>[4x]MRIQVNAKGAARLLSRHLWVFRRDVVSGPETPGLYPVYWGRRFLALALYNPHTDLAVRAYRFAPA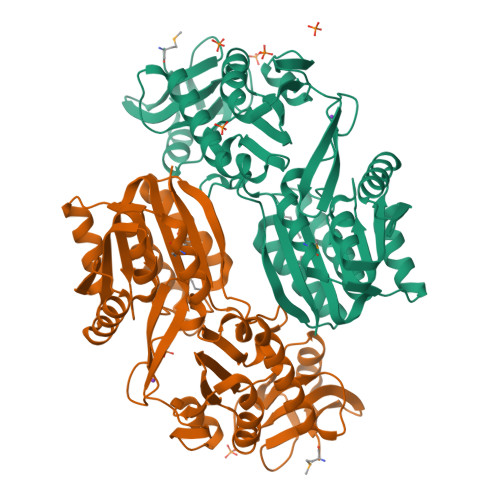EDPVAALLENLAQALARREAVLRQDPEGGYRLVHAEGDLLPGLVVDYYAGHAVVQATAHAWEGLLPQVAEALRPHVQSVLAKNDARTRELEGLPLYVRPLLGEVPERVQVQEGRVRYLVDLRAGQKTGAYLDQRENRLYMERFRGERALDVFSYAGGFALHLALGFREVVAVDSSAEALRRAEENARLNGLGNVRVLEANAFDLLRRLEKEGERFDLVVLDPPAFAKGKKDVERAYRAYKEVNLRAIKLLKEGGILATASCSHHMTEPLFYAMVAEAAQDAHRLLRVVEKRGQPFDHPVLLNHPETHYLKFAVFQVL> GAGCAGCCTGT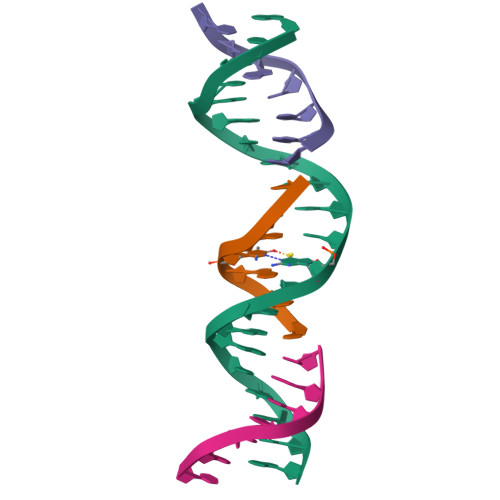GTGGACATCA;> CCACACA;> GGCTGCT;> CTGATGT> GSMSAKDERAREILRGFKLNWMNLRDAETGKILWQGTEDLSVPGVEHEARVPKKILKCKAVSRELNFSSTEQMEKFRLEQKVYFKGQCLEEWFFEFGFVIPNSTNTWQSLIEAAPESQMMPASVLTGNVIIETKF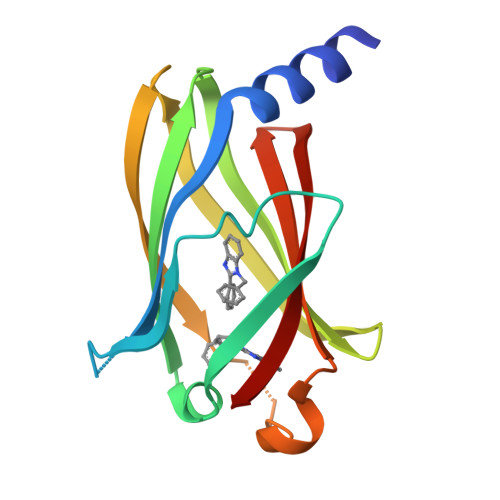FDDDLLVSTSRVRLFYV> MKSSHHHHHHENLYFQSNASEFFWDVQKIQEISNVEEHSVVKCVTVNTSRLISQLNEELQDEESGVNFIVTQLQLLINNVYEKIQKSPGVPAHRSLMINLNFTRLKFSIAYWDILLERSLDLINGPSKTGARYFITEVT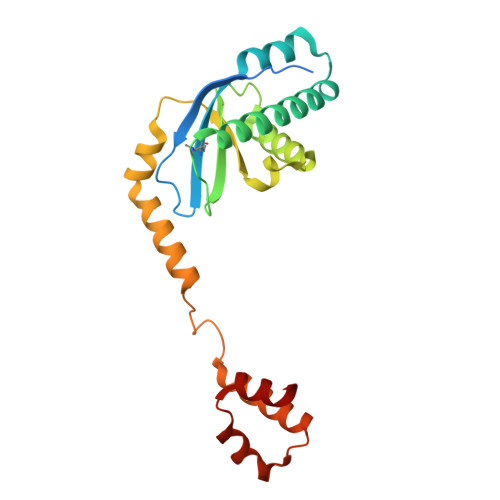PVDRSRYVENNQYFLAFKANQRLTRNSVDMDEFIDFEILIKQIIFDLFKKNGIPDQDFEAILSRFHNLESLVVAFNE> QLPPSLPSDPRLWSREDVLVFLRFCVREFDLPKLDF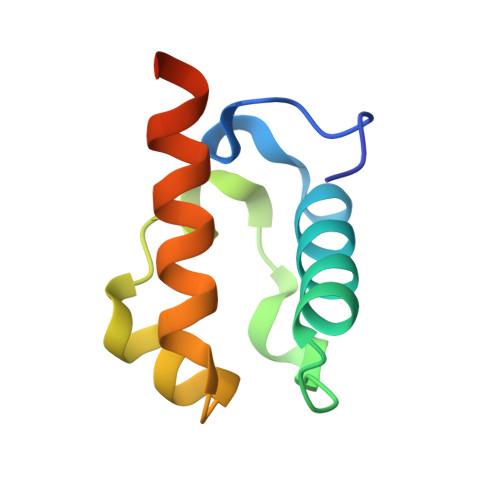DLFQMNGKRLCLLTRADFGHRCPGAGDVLHNVLQMLIIESHSRHHHHHH> MLTEGISIQSYDGHTFGALVGSPAKAPAPVIVIAQEIFGVNAFMRETVSWLVDQGYAAVCPDLYARQAP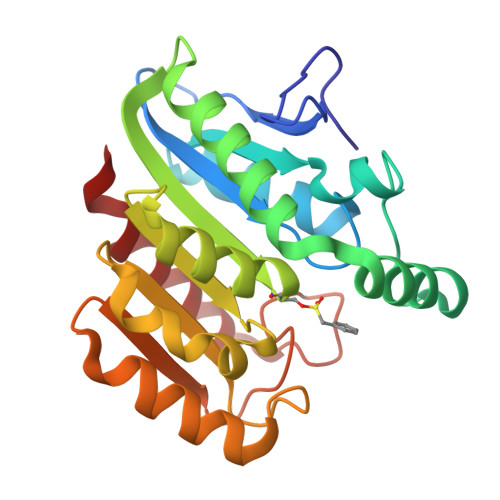GTALDPQDEAQREQAYKLWQAFDMEAGVGDLEAAIRYARHQPYSNGKVGLVGYSLGGALAFLVAAKGYVDRAVGYYGVGLEKQLNKVPEVKHPALFHMGGQDHFVPAPSRQLITEGFGANPLLQVHWYEEAGHSFARTSSSGYVASAAALANERTLDFLAPLQ> MRGSHHHHHHGSVHPDLRDVFSKMSFFDKIGFLFIHAFDKRNLWHKVPVPIGLLYLNTRRTLLEKYNLLAVGRSSHGALFDPKEFLYRTEDGKYNDPHNAEAGSQNTFFGRNMEPVDQQDELMSPDPFVVATKLLARREYKDTGKQFNILAAAWIQFMVHDWMDHMEDTGQIGITAPKEVANECPLKSFKFHPTKELPTNSDGIKIGHYNIRTAWWDGSAVYGNNEERAEKLRTYVDGKLVIGDDGLLLHKENGVALSGDIRNSWAGVSILQALFVKEHNAVCDAIKEEHPNLSDEELYRYAKLVTSAVIAKVHTIDWTVELLKTKTMRAAMRANWYGLLGKKIKDTFGHIGGPILGGLVGLKKPNNHGVPYSLTEEFTSVYRMHSLIPSTLKLRDPTGQPDANNSPPCLEDIDIGEMIGLKGEEQLSKIGFEKQALSMGYQACGALELWNYPSFFRNLIPQNLDGTNRSDRIDLAALEVYRDRERSVPRYNEFRRRLFLIPIKSWEDLTSDKDAIETIRAIYGDDVEKLDLLVGLMA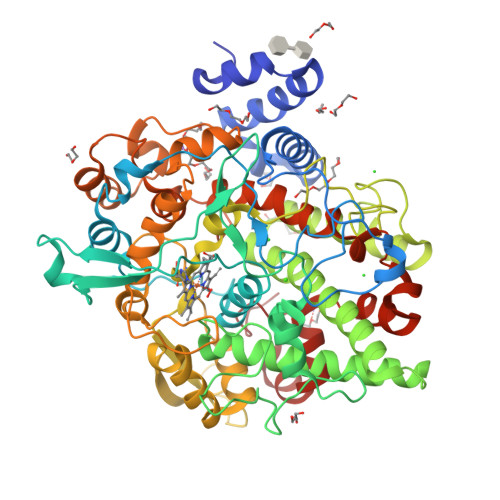EKKIKGFAISETAFNIFILMASRRLEADRFFTSNFNEETYTKKGMQWVKTTEGLRDVINRHYPEITAKWMKSSSAFSVWDADY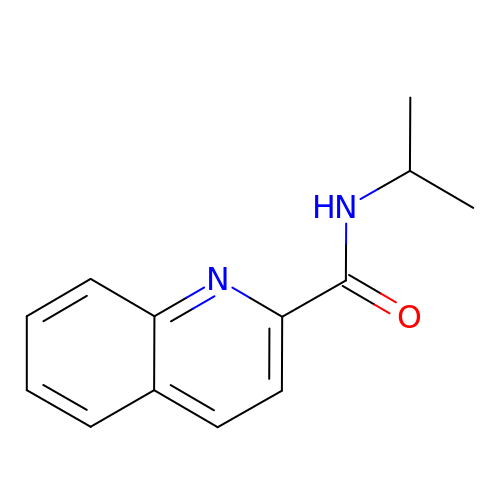~{N}-propan-2-ylquinoline-2-carboxamide | C13 H14 N2 O | MWZFFJAEAZQGLX-UHFFFAOYSA-N> MAIETNAVVITDLNPLYPRDRDYIYEGAAQIRLIKQTLQNTFPNVTEPVDIDSDTFKIMSEKLKFTGDAMDVGGLMIKNVTPGTGDKDVVTKGQMEAFMKNWMENKLYRIGSYYITEEDINPGDSISLGFGSWAKVTGVIMGTGVVNPDGSVPNAQRVEFQAGGTGGRVFNTIRTENVPLMTVNGSSFSLSSNTHSHNMVFGRGDASGHNSSPNWYSPGGGYSQRTDNDTHTHTISGSVSLGRDDISRQPIN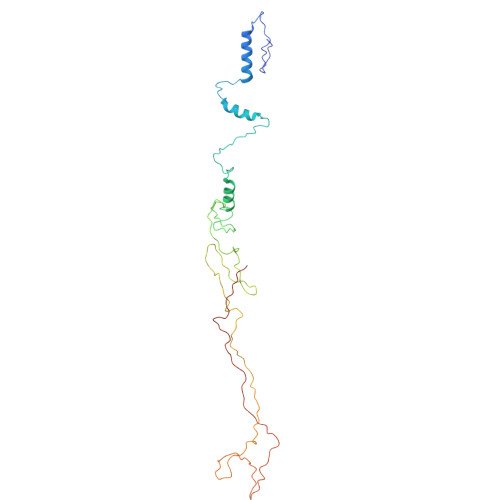TLPPFRAAHIWRRIS> MNPKSLTRGP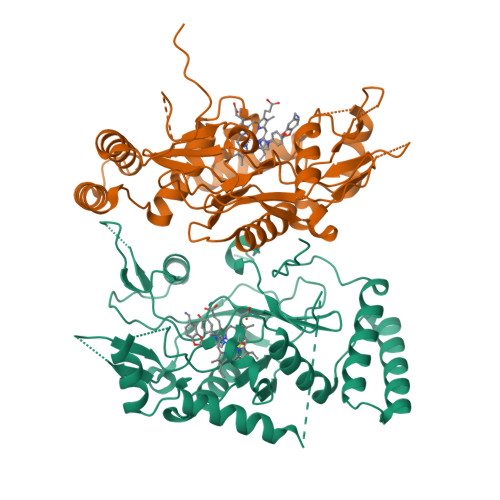RDKPTPLEELLPHAIEFINQYYGSFKEAKIEEHLARLEAVTKEIETTGTYQLTLDELIFATKMAWRNAPRCIGRIQWSNLQVFDARNCSTAQEMFQHICRHILYATNNGNIRSAITVFPQRSDGKHDFRLWNSQLIRYAGYQMPDGTIRGDAATLEFTQLCIDLGWKPRYGRFDVLPLVLQADGQDPEVFEIPPDLVLEVTMEHPKYEWFQELGLKWYALPAVANMLLEVGGLEFPACPFNGWYMGTEIGVRDFCDTQRYNILEEVGRRMGLETHTLASLWKDRAVTEINVAVLHSFQKQNVTIMDHHTASESFMKHMQNEYRARGGCPADWIWLVPPVSGSITPVFHQEMLNYVLSPFYYYQIEPWKTHIWQNEHHHH> MSGGDGRGHNTGAHSTSGNINGGPTGLGVGGGASDGSGWSSENNPWGGGSGSGIHWGGGSGHGNGGGNGNSGGGSGTGGNLSAVAAPVAFGFPALSTPGAGGLAVSISAGALSAAIADIMAALKGPFKFGLWGVALYGVLPSQIAKDDPNMMSKIVTSLPADDITESPVSSLPLDKATVNVNVRVVDDVKDERQNISVVSGVPMSVPVVDAKPTERPGVFTASIPGAPVLNISVNNSTPAVQTLSPGVTNNTDKDVRPAFGTQGGNTRDAVIRFPKDSGHNAVYVSVSDVLSPDQVKQRQDEENRRQQEWDATHPVEAAERNYERARAELNQANEDVARNQERQAKAVQVYNSRKSELDAANKTLADAIAEIKQFNRFAHDPMAGGHRMWQMAGLKAQRAQTDVNNKQAAFDAAAKEKSDADAALSSAMESRKKKEDKKRSAENNLNDEKNKPRKGFKDYGHDYHPAPKTENIKGLGDLKPGIPKTPKQNGG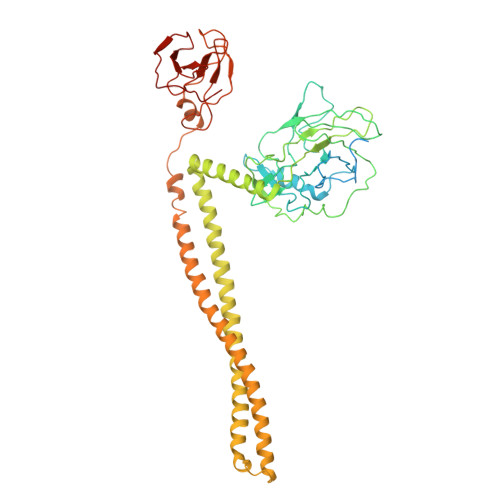GKRKRWTGDKGRKIYEWDSQHGELEGYRASDGQHLGSFDPKTGNQLKGPDPKRNIKKYL>GNFKEADDAIHYRQSAFSLMAHNFGDMGAML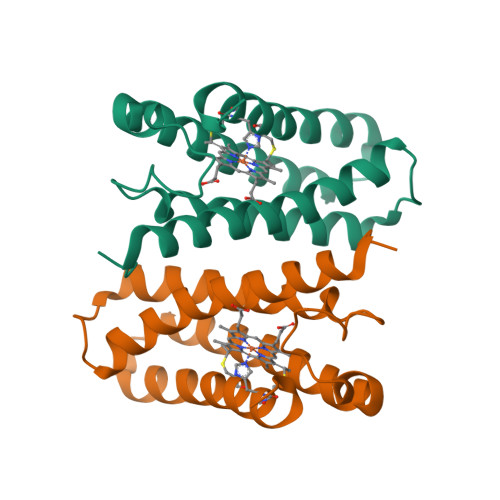KGKKPFDSEIFTMRAENVAALSKLPLEGFIQGSDLGDTEALAKIWTDKSDFDAKMVSLQDNAAALLLASASDDKKLLKQSFMKVAKSCKGCHDVYKKD[2x]>MVEVLADHPGELVRTDSPNFLCSVLPTHWRCNKTLPIAFKVVALGDVP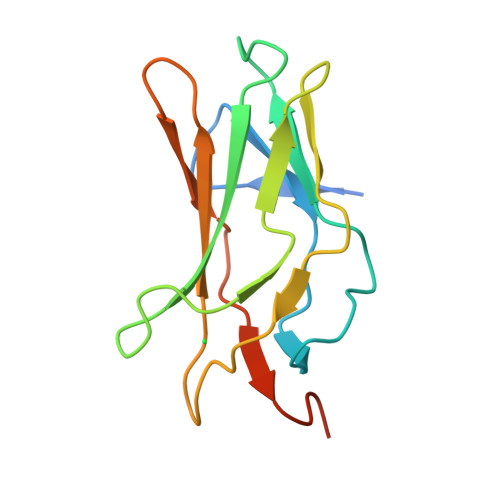DGTLVTVMAGNDENYSAELRNATAAMKNQVARFNDLRFVGRSGRGKSFTLTITVFTNPPQVATYHRAIKITVDGPREPRRHRQ[2x]>[2x]MAVEEIVKVSRNYQVTIPAKVRQKFQIKEGDLVKVTFDESEGVVKIQLLKEPWK

Sso7c4 appears to be the first repressor-like protein described in crenarchaea and may play a regulatory role in gene transcription. The Sso7c4 protein possesses a homodimeric DNA-binding fold that forms a swapped β-loop-β ‘Yin-Yang’ topology, and it belongs to the SpoVT-AbrB superfamily. The dimeric Sso7c4 protein, which consists of eight intertwined β sheets and two flanking α helices, forms a dimer via intermolecular associations between β1 and β3′ (the primes indicate the second monomer in the dimer) and β1′ and β3 in the flank, β2 and β2′ at the top, and β4 and β4′ at the bottom. In our study, Sso7c4 exhibits DNA-binding activity and alters the trajectory of the DNA through bending and bridging.

Here, we present the crystal structure of wild-type Sso7c4, which was resolved at a high resolution of 1.63 Å, to obtain a better understanding of its architectural properties and functions. The crystal of wild-type Sso7c4 contains one homodimer in the asymmetric unit and is in the P212121 space group. Interestingly, the two basic C-termini are disordered owing to a lack of corresponding density. In the wild-type crystal, Sso7c4 makes extensive contacts with neighboring molecules via residues in loop1 (R11, N12, and Y13), the α1 helix (K20, R22, and K24), loop3 (E29) and loop4 (E39). Three sulfate ions, which all bind to the top surface of wild-type Sso7c4, are present in the crystal structure. Two (X201 and X202) are located near the R22 (R22′) side chains, mediate protein-protein interactions, and are solvated by eight water molecules; the third (X203) is close to the β2′ strand on the DNA-binding surface. We believe that the relative positions of these three sulfates on the top surface of Sso7c4 mimic the position of the phosphate backbone of DNA upon complex formation. In contrast, the R11 side chains in the wild-type Sso7c4 crystal structure are stabilized by intermolecular interactions. In addition, the R11 side chain (chain A) of the wild-type protein is further stabilized by PEG 400 through water-mediated hydrogen bonds. The K24 side chain is more ordered in chain A, which is stabilized by polyethylene glycol 400 (PEG 400), similar to the stabilization observed in crown ether binding mode.UvrD is classified as a SF1A helicase and plays important functions in DNA replication, recombinational repair, methyl-directed mismatch repair and nucleotide excision repair. UvrD consists of two RecA-like domains (1A and 2A) that are responsible for nucleotide binding and hydrolysis and two additional domains (1B and 2B) that are involved in dsDNA binding. Here we present crystal structures of full-length and a C-terminally truncated construct of D. radiodurans UvrD (drUvrD) in complex with 3′-tailed dsDNA. Our structures obtained in apo- and AMPPNP bound states provide us with several snapshots of this essential cellular process and reveal a large-scale spiral movement of UvrD around the duplexed DNA.

Crystal form I appeared very rapidly (<1 day) and belonged to space group P212121 with two protein monomers and one DNA duplex per asymmetric unit, while crystal form II appeared after at least one week and belonged to space group P21 with four molecules of protein and two DNA duplexes per asymmetric unit. In the structures of drUvrDFL and drUvrD∆C form I, each protein monomer contains one bound AMPPNP molecule, whereas in drUvrD∆C form II each assembly is composed of a DNA duplex with an AMPPNP-bound UvrD on one end and an apo-UvrD on the other. In drUvrD∆C, loss of one of the AMPPNP molecules leads to the formation of crystal form II in which the apo molecule has rotated 125° around the DNA with respect to the position of drUvrDFL or 105° with respect to crystal form I, resulting in an assembly with one drUvrD on either side of the DNA duplex. In this assembly, the apo-drUvrD∆C molecule has twisted the 3′-ssDNA extension and maintains the ssDNA in a bent orientation with respect to the DNA duplex axis. As a result, the DNA duplex itself shows a reduced helical twist and reduced bending. The loss of the bound nucleotide also results in major structural rearrangements within the protein monomer. Loss of the nucleotide induces a ~15° rotation of domain 2B and an ~8° rotation of domains 1A and 1B relative to domain 2A in the plane formed by the ss- and dsDNA. In the AMPPNP-bound molecule of drUvrD∆C form II, nucleotides 20 to 23 are bound in the binding pocket, indicating that drUvrD has translocated along the ssDNA by one nucleotide compared to form I and as a result both nucleotides 24 and 25 have become untraceable. As in ecUvrD, the apo-drUvrD∆C observed in crystal form II, reveals a fifth nucleotide in the ssDNA binding pocket. In the absence of nucleotide, however, only two of these contacts remain: the GIG sequence in the α17-α18 HLH motif interacts with nt7-10 and Phe633 from the β-hairpin motif stacks against the first base-pair.

>[4x]MTSSAGPDLLQALNPTQAQAADHFTGPALVIAGAGSGKTRTLIYRIAHLIGHYGVHPGEILAVTFTNKAAAEMRERAGHLVPGAGDLWMSTFHSAGVRILRTYGEHIGLRRGFVIYDDDDQLDIIKEVMGSIPGIGAETQPRVIRGIIDRAKSNLWTPDDLDRSREPFISGLPRDAAAEAYRRYEVRKKGQNAIDFGDLITETVRLFKEVPGVLDKVQNKAKFIHVDEYQDTNRAQYELTRLLASRDRNLLVVGDPDQSIYKFRGADIQNILDFQKDYPDAKVYMLEHNYRSSARVLEAANKLIENNTERLDKTLKPVKEAGQPVTFHRATDHRAEGDYVADWLTRLHGEGRAWSEMAILYRTNAQSRVIEESLRRVQIPARIVGGVGFYDRREIRDILAYARLALNPADDVALRRIIGRPRRGIGDTALQKLMEWARTHHTSVLTACANAAEQNILDRGAHKATEFAGLMEAMSEAADNYEPAAFLRFVMETSGYLDLLRQEGQEGQVRLENLEELVSAAEEWSQDEANVGGSIADFLDDAALLSSVDDMRTKAENKGAPEDAVTLMTLHNAKGLEFPVVFIVGVEQGLLPSKGAIAEGPSGIEEERRLFYVGITRAMERLLMTAAQNRMQFGKTNAAEDSAFLEDIEGLFDTVDPYGQPIEYR>[2x]MSTENVEGKPSNLGERGRARSSTFLRVVQPMFNHSIFTSAVSPAAERIRFILGEEDDSPAPPQLFTELDELLAVDGQEMEWKETARWIKFEEKVEQGGERWSKPHVATLSLHSLFELRTCMEKGSIMLDREASSLPQLVEMIVDHQIETGLLKPELKDKVTYTLLRKHRHQTKKSNLRSLADIGKTVSSASRMFTNPDNGSPAMTHRNLTSSSLNDISDKPEKDQLKNKFMKKLPRDAEASNVLVGEVDFLDTPFIAFVRLQQAVMLGALTEVPVPTRFLF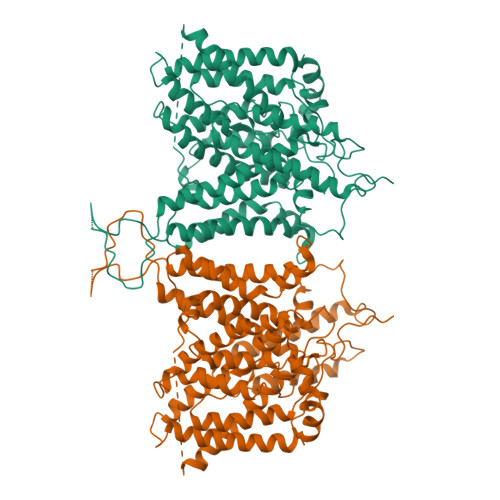ILLGPKGKAKSYHEIGRAIATLMSDEVFHDIAYKAKDRHDLIAGIDEFLDEVIVLPPGEWDPAIRIEPPKSLPSSDKRKNMYSGGENVQMNGDTPHDGGHGGGGHGDCEELQRTGRFCGGLIKDIKRKAPFFASDFYDALNIQALSAILFIYLATVTNAITFGGLLGDATDNMQGVLESFLGTAVSGAIFCLFAGQPLTILSSTGPVLVFERLLFNFSKDNNFDYLEFRLWIGLWSAFLCLILVATDASFLVQYFTRFTEEGFSSLISFIFIYDAFKKMIKLADYYPINSNFKVGYNTLFSCTCVPPDPANISISNDTTLAPEYLPTMSSTDMYHNTTFDWAFLSKKECSKYGGNLVGNNCNFVPDITLMSFILFLGTYTSSMALKKFKTSPYFPTTARKLISDFAIILSILIFCVIDALVGVDTPKLIVPSEFKPTSPNRGWFVPPFGENPWWVCLAAAIPALLVTILIFMDQQITAVIVNRKEHKLKKGAGYHLDLFWVAILMVICSLMALPWYVAATVISIAHIDSLKMETETSAPGEQPKFLGVREQRVTGTLVFILTGLSVFMAPILKFIPMPVLYGVFLYMGVASLNGVQFMDRLKLLLMPLKHQPDFIYLRHVPLRRVHLFTFLQVLCLALLWILKSTVAAIIFPVMILALVAVRKGMDYLFSQHDLSFLDDVIPEKDKKKKEDEKKKKKKKGSLDSDNDDSDCPYSEKVPSIKIPMDIMEQQPFLSDSKPSDRERSPTFLERHTSC> GGIAIYWGQNGNEGTLTQTCSTRKYSYVNIAFLNKFGNGQTPQINLAGHCNPAAGGCTIVSNGIRSCQIQGIKVMLSLGGGIGSYTLASQADAKNVADYLWNNFLGGKSSSRPLGDAVLDGIDFAIAHGSTLYWDDLARYLSAYSKQGKKVYLTAAPQCPFPDRYLGTALNTGLFDYVWVQFFNNPPCQYSSGNINNIINSWNRW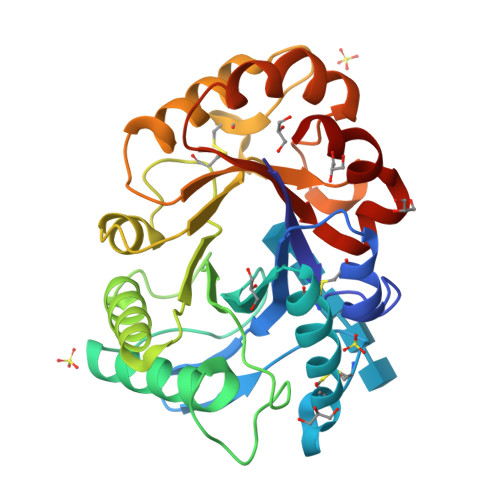TTSINAGKIFLGLPAAPEAAGSGYVPPDVLISRILPEIKKSPKYGGVMLWSKFYDDKNGYSSSILDSV> MKIAVIGQSLFGQEVYKELKNEGHMIVGVFTIPDKDGKVDPLAIEAEKDGVPVFKFPRWRLKGKAITEVVDQYKAVGAELNVLPFCSQFIPMEVIDHPKHGSIIYHPSLLPRHRGASAINWTLIHGDKKGGFTVFWADDGLDTGPILLQRECDVEPNDNVNSIYKRFLFPEGVKGMVEAVRLIATGKAPRIKQPEEGATAECIQKKENSKIDWNQPAEAIHNWIRGNDRVPGAWAEIDGKSVSFYGSTLLENDHFSSNGQPLEIPGASRAALVTKNGLVLFGNDGKMLLVKNLQFEDGKMIPG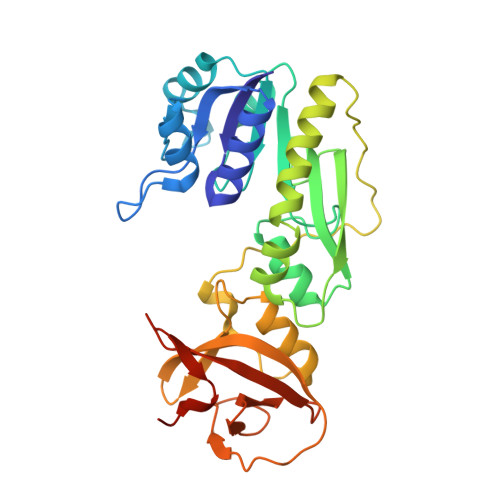SQYFKAGVEHHHHHH4-(4-pyrrol-1-ylphenyl)morpholine 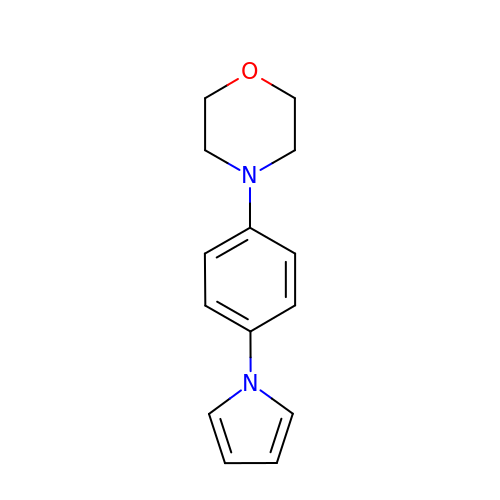| C14 H16 N2 O | VJGOAQUQJGASLY-UHFFFAOYSA-N>[3x]PTLEVFLPAGHDDARKAELIARLTGATVDSIG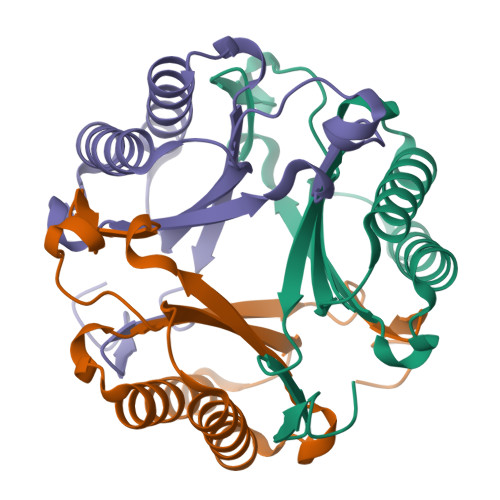APIESVRVLLTELPATHIGLGGRSAADGAPPSLPVIVAILIAGRTDEQKRALIAALSETSASVLDAPLQATRVMIKDIPNTDFGIGGQTARALGR> MSADSSPLVGSTPTGYGTLTIGTSIDPLSSSVSSVRLSGYCGSPWRVIGYHVVVWMMAGIPLLLFRWKPLWGVRLRLRPCNLAHAETLVIEIRDKEDSSWQLFTVQVQTEAIGEGSLEPSPQSQAEDGRSQAAVGAVPEGAWKDTAQLHKSEEAVSVGQKRVLRYYLFQGQRYIWIETQQAFYQVSLLDHGRSCDDVHRSRHGLSLQDQMVRKAIYGPNVISIPVKSYPQLLVDEALNPYYGFQAFSIALWLADHYYWYALCIFLISSISICLSLYKTRKQSQTLRDMVKLSMRVCVCRPGGEEEWVDSSELVPGDCLVLPQEGGLMPCDAALVAGECMVNESSLTGESIPVLKTALPEGLGPYCAETHRRHTLFCGTLILQARAYVGPHVLAVVTRTGFCTAKGGLVSSILHPRPINFKFYKHSMKFVAALSVLALLGTIYSIFILYRNRVPLNEIVIRALDLVTVVVPPALPAAMTVCTLYAQSRLRRQGIFCIHPLRINLGGKLQLVCFDKTGTLTEDGLDVMGVVPLKGQAFLPLVPEPR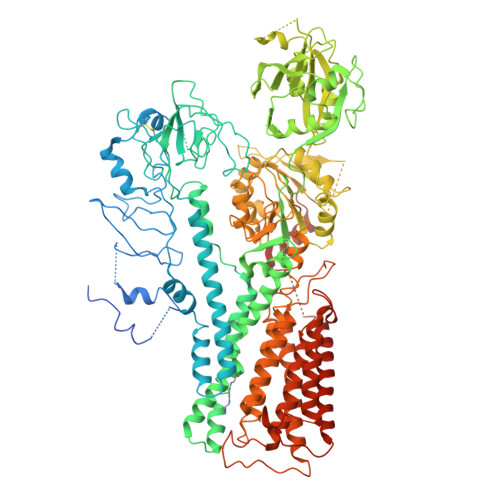RLPVGPLLRALATCHALSRLQDTPVGDPMDLKMVESTGPQLQAMEEPPVPVSVLHRFPFSSALQRMSVVVAWPGATQPEAYVKGSPELVAGLCNPETVPTDFAQMLQSYTAAGYRVVALASKPLPTVPSLEAAQQLTRDTVEGDLSLLGLLVMRNLLKPQTTPVIQALRRTRIRAVMVTGDNLQTAVTVARGCGMVAPQEHLIIVHATHPERGQPASLEFLPMESPTAVNGVKDPDQAASYTVEPDPRSRHLALSGPTFGIIVKHFPKLLPKVLVQGTVFARMAPEQKTELVCELQKLQYCVGMCGDGANDCGALKAADVGISLSQAEASVVSPFTSSMASIECVPMVIREGRCSLDTSFSVFKYMALYSLTQFISVLILYTINTNLGDLQFLAIDLVITTTVAVLMSRTGPALVLGRVRPPGALLSVPVLSSLLLQMVLVTGVQLGGYFLTLAQPWFVPLNRTVAAPDNLPNYENTVVFSLSSFQYLILAAAVSKGAPFRRPLYTNVPFLVALALLSSVLVGLVLVPGLLQGPLALRNITDTGFKLLLLGLVTLNFVGAFMLESVLDQCLPACLRRLRPKRASKKRFKQLERELAEQPWPPLPAGPLR>ALTGSRPSVVYLHAAECTGCSEALLRTYQPFIDTLILDTISLDYHETIMAAAGEAAEEALQAAVNGPDGFICLVEGAIPTGMDNKYGYIAGHTMYDICKNILPKAKAVVSIGTCACYGGIQAAKPNPTAAKGINDCYADLGVKAINVPGCPPNPLNMVGTLVAFLKGQKIELDEVGRPVMFFGQSVHDLCERRKHFDAGEFAPSFNSEEARKGWCLYDVGCKGPETYNNCPKVLFNETNWPVAAGHPCIGCSEPNFWDDMTPFYQN[2x];>SQVTKTPRSNYTGPIVVDPLTRIEGHLRIEVEVEGGVIKEARSCATLFRGIETILKGRDPRDAQHFTQRTCGVCTYTHALASTRCLEDAINKPIPANATYIRNLVLGNQFMHDHLVHFYHLHALDFVDVTSALLADPAKAAKLANSISPRKATTEEFAAVQAKLKTFVASGQLGPFTNAYFLGGHEGYYMDPEANLVCTAHYLQALRAQVEVAKGMAVFGAKNPHTQFTVAGGVTCYEALTPERIKQFRELYVKARAFIEEVYIPDLLLVASYYKDWGKIGGTNNFMAFGEFPAPGGERDLNSRWYKPGVIYDRKVGSVQPFDPSKIEE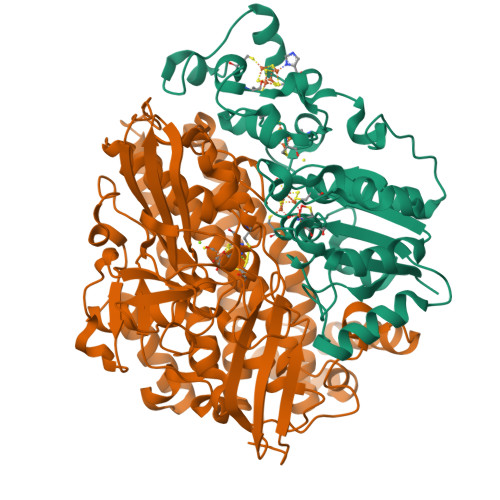HVRHSWYEGKARAPFEGETNPHFTFMGDTDKYSWNKAPRYDGHAVETGPLAQMLVAYGHNHKTIKPTIDAVLGKLNLGPEALFSTLGRTAARGIQTLVIAQQMENWLNEYENNIVKDKQIVEDYAVPTSARGVGFADVSRGGLSHWMTIEDGKIDNFQLVVPTTWNLGPRDDKGVPSAAEAALVGTPVADPKRPVEILRTIHSFDPCIACSTH[2x]>[8x]MGLTIGVDIGGTKIAAGVVDEEGRILSTFKVATPPTAEGIVDAICAAVAGASEG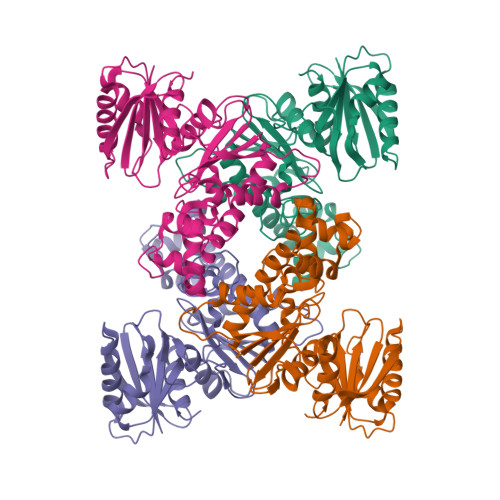HDVEAVGIGAAGYVDDKRATVLFAPNIDWRHEPLKDKVEQRVGLPVVVENDANAAAWGEYRFGAGQGHDDVICITLGTGLGGGIIIGNKLRRGRFGVAAEFGHIRVVPDGLLCGCGSQGCWEQYASGRALVRYAKQRANATPENAAVLLGLGDGSVDGIEGKHISEAARQGDPVAVDSFRELARWAGAGLADLASLFDPSAFIVGGGVSDEGELVLDPIRKSFRRWLIGGEWRPHAQVLAAQLGGKAGLVGAADLARQGLEHHHHHH>[4x]MSPFHLNDAVAIVTGAAAGIGRAIAGTFAKAGASVVVTDLKSEGAEAVAAAIRQAGGKAIGLECNVTDEQHREAVIKAALDQFGKITVLVNNAGGGGPKPFDMPMSDFEWAFKLNLFSLFRLSQLAAPHMQKAGGGAILNISSMAGENTNVRMASYGSSKAAVNHLTRNIAFDVGPMGIRVNAIAPGAIKTDALATVLTPEIERAILKHTPLGRLGEAQDIANAALFLCS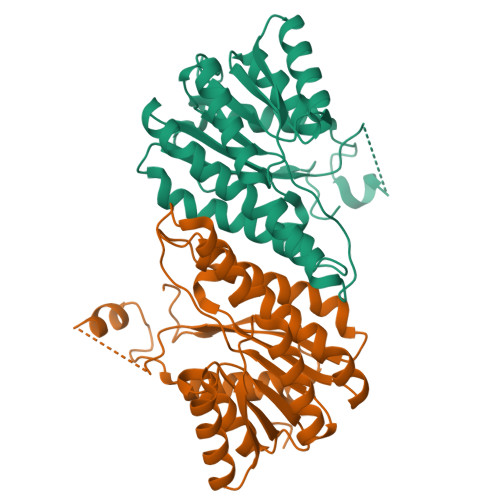PAAAWISGQVLTVSGGGVQELD>[3x]MANLAAGQSYVRNVALALEAQRDPSTGALPTHLTDCLSGFGQRP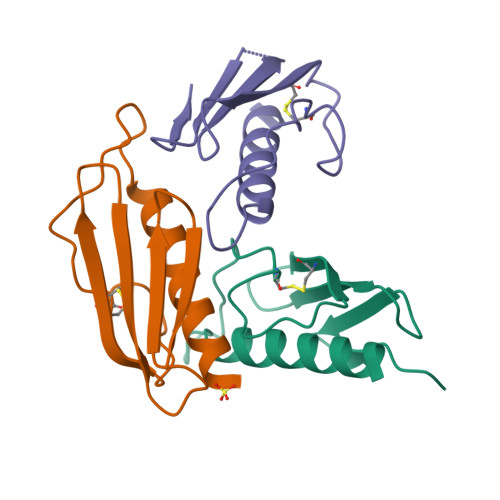KTVTACTITYLNALDYVIEASLDGAALKKVVYKSSDGTLTSLPLEHHHHHH>STHFDVIVVGAGSMGMAAGYQLAKQGVKTLLVDAFDPPHTNGSHHGDTRIIRHAYGEGREYVPLALRSQELWYELEKETHHKIFTKTGVLVFGPKGESAFVAETMEAAKEHSLTVDLLEGDEINKRWPGITVPENYNAIFEPNSGVLFSENCIRAYRELAEARGAKVLTHTRVEDFDISPDSVKIETANGSYTADKLIVSMGAWNSKLLSKLNLDIPLQPYRQVVGFFESDESKYSNDIDFPGFMVEVPNGIYYGFPSFGGCGLKLGYHTFGQKIDPD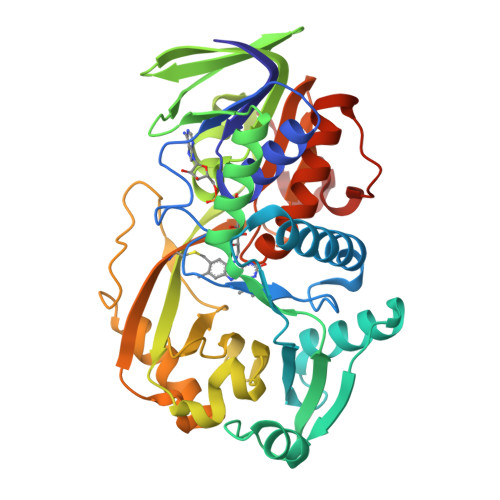TINREFGVYPEDESNLRAFLEEYMPGANGELKRGAVCMYTKTLDEHFIIDLHPEHSNVVIAAGFSGHGFKFSSGVGEVLSQLALTGKTEHDISIFSINRPALKESLQKTTI[2x]>MGFLDGKRILLTGLLSNRSIAYGIAKACKREG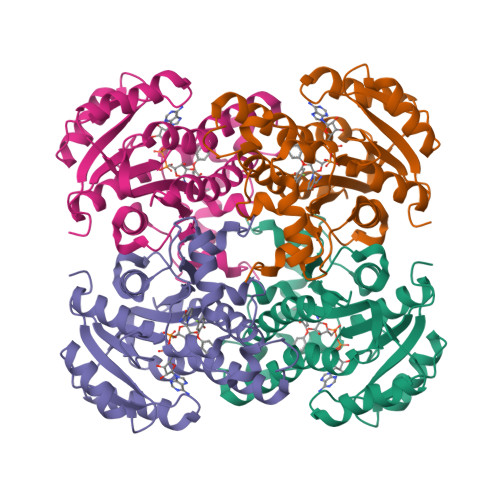AELAFTYVGDRFKDRITEFAAEFGSELVFPCDVADDAQIDALFASLKTHWDSLDGLVHSIGFAPREAIAGDFLDGLTRENFRIAHDISAYSFPALAKAALPMLSDDASLLTLSYLGAERAIPNYNTMGLAKAALEASVRYLAVSLGAKGVRVNAISAGPIKTLAASGIKSFGKILDFVESNSPLKRNVTIEQVGNAGAFLLSDLASGVTAEVMHVDSGFNAVVGGMAGLEEKLAAALEHHHHHH[12x]> MVGQVIR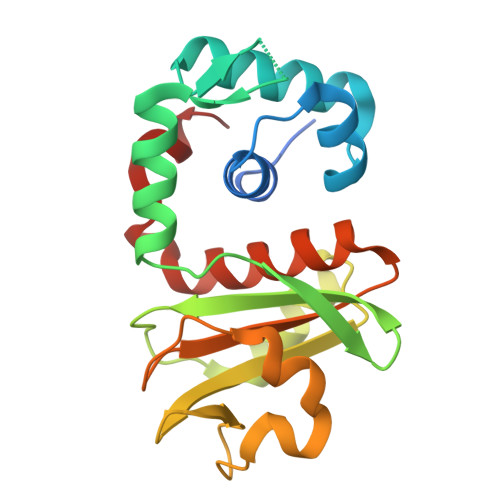KRGAYPEYTVEDVLAVIFLLKEPLGRKQISERLELGEGSVRTLLRKLSHLDIIRSKQRGHFLTLKGKEIRDKLLSMFSEPIGVSVDGYPGIAIVVKNPPEFKSIELRDEAIKFDAKGAMILTVKDNEIVFPEDFRPLKEMYPEVAKKIVDYEDGDAVIITWAETPAKALKSAIHVAYILKKEEITPEILEVVK> MRCIGISNRDFVEGVSGGSWVDIVLEHGSCVTTMAKNKPTLDFELIKTEAKHPATLRKYCIEAKLTNTTTASRCPTQGEPSLNEEQDKRFVCKHSMVDRGWGNGCGLFGKGGIVTCAMFTCKKNMEGKVVQPENLEYTIVITPHSGEENAVGNDTGKHGKEIKVTPQSSITE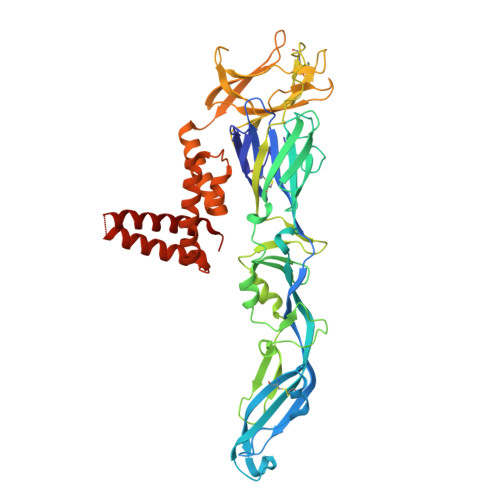AELTGYGTVTMECSPRTGLDFNEMVLLQMENKAWLVHRQWFLDLPLPWLPGADTQGSNWIQKETLVTFKNPHAKKQDVVVLGSQEGAMHTALTGATEIQMSSGNLLFTGHLKCRLRMDKLQLKGMSYSMCTGKFKVVKEIAETQHGTIVIRVQYEGDGSPCKIPFEIMDLEKRHVLGRLITVNPIVTEKDSPVNIEAEPPFGDSYIIIGVEPGQLKLSWFKKGSSIGQMFETTMRGAKRMAILGDTAWDFGSLGGVFTSIGKALHQVFGAIYGAAFSGVSWTMKILIGVVITWIGMNSRSTSLSVSLVLVGVVTLYLGVMVQA>[2x]SMNPFMNTNPFLEELDQPIPSNAAKPISEETRDLFLSDGQTIPSSQEKIATIHEYLLEHKELEEAMFSLISQGRGRSLINMVVKSALNIETQSREVTGERRQRLERKLRNLENQGIYVDESKIMSRGRISKEDTELAMRIARKNQKDAKLRRIYSNNASIQESYTVDDFVSYWMEQESLPTGIQIAMWLKGDDWSQPIPPRVQRRHYDSYIMMLGPSPTQEQADAVKDLVDDIYDRNQG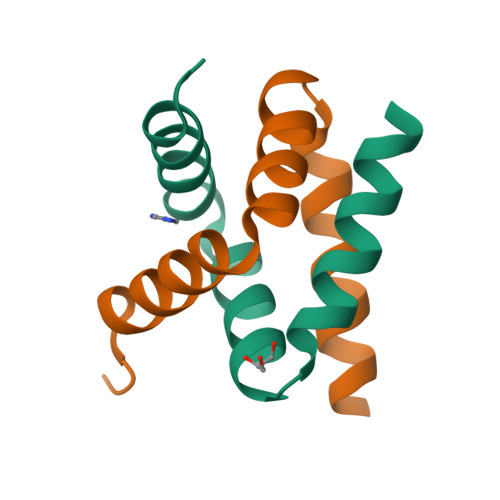KGPSQEQARELSHAVRRLISHSLVNQPATAPRVPPRRIVSAQTAQTDPPGRRAALDRLRRVRGEDNDIV> MREYKLVVLGSGGVGKSALTVQFVQGIFVDEYDPTIEDSYRKQVEVDCQQCMLEILDTAGTEQFTAMRDLYMK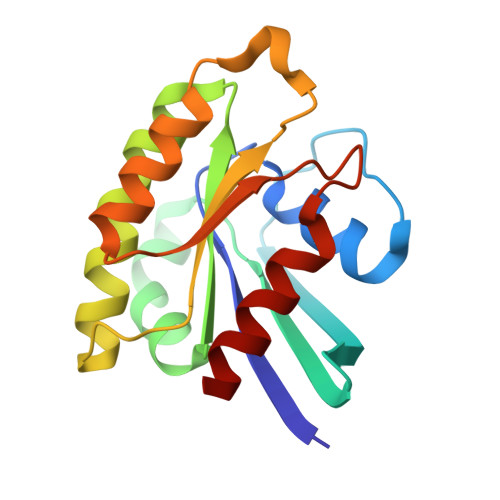NGQGFALVYSITAQSTFNDLQDLREQILRVKDTEDVPMILVGNKCDLEDERVVGKEQGQNLARQWCNCAFLESSAKSKINVNEIFYDLVRQINR>[2x]ASSRWFFTREQLENTPSRRCGVEADKELSCRQQAANLIQEMGQRLNVSQLTINTAIVYMHRFYMHHSFTKFNKNIISSTALFLAAKVEEQARKLEHVIK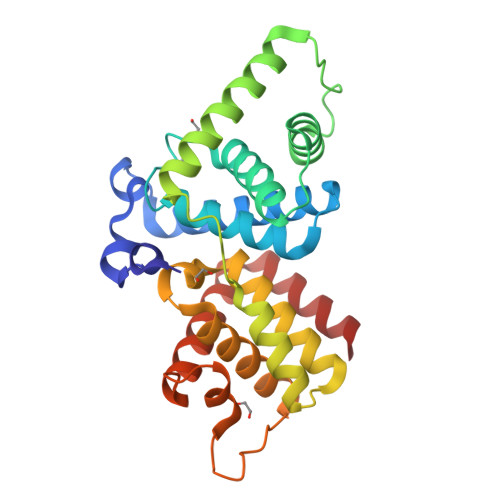VAHACLHPLEPLLDTKCDAYLQQTRELVILETIMLQTLGFEITIEHPHTDVVKCTQLVRASKDLAQTSYFMATNSLHLTTFCLQYKPTVIACVCIHLACKWSNWEIPVSTDGKHWWEYVDPTVTLELLDELTHEFLQILEKTPNRLKKIRNWRANQAA ALPHA-KETOMALONIC ACID | C3 H2 O5 | 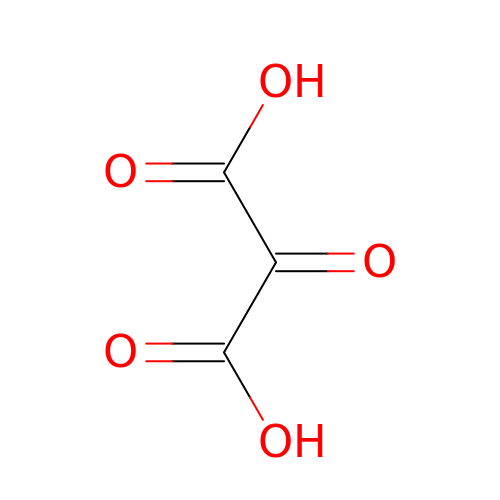XEEVLJKYYUVTRC-UHFFFAOYSA-N> SPSAFPYFHPTKEIFIPGQVRNLIEMCQVDTLIPVNNTQENVRSVNMYTVDLRTQVDLAKEVFSI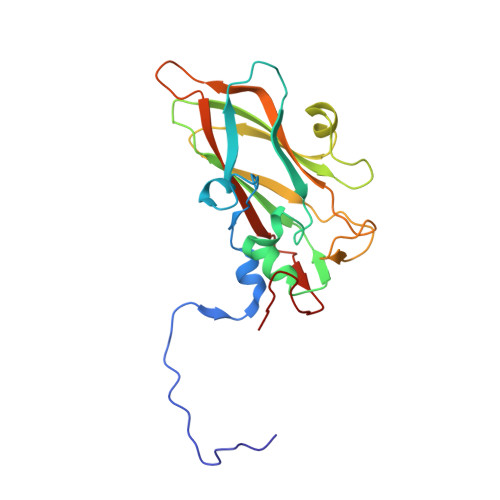PVDIASQPLATTLIGELASYYTHWTGSLRFSFMFCGSASSTLKLLIAYTPPGVGKPKSRREAMLGTHLVWDVGLQSTASLVVPWVSASHFRFTTPDTYSSAGYITCWYQTNFVVPDSTPDNAKMVCMVSACKDFCLRLARDTNLHTQEG> GPSPDTCSQDLNSRVKPGFPKTIKTNDPGVLQAARYSVEKFNNCTNDMFLFKESRITRALVQIVKGLKYMLEVEIGRTTCKKNQHLRLDDCDFQTNHTLKQTLSCYSEVWV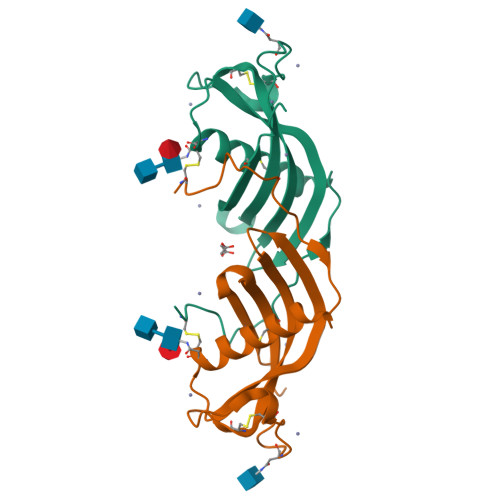VPWLQHFEVPVLRCHHHHHH>MRLQKDFDRVMGIILMILILAIPSLQICNKSYTEGDPVIINPVPGLPVDFIRGVDASEAPWIIELGGKYYDENGVERDLLDILKENGVNWIRLRVWNDPYDEQGRPYGGGNCDLPRMTDFAAKAKAKGFGVLIDFHYSDWWADPSKQSKPKAWANLSYPELVEAVYNWTYNALKYMAEHNALPDMVQIGNEINNGFLWPDGSAANWTQFVGLLKAAISAVKDVNPNIKIVIHLAGVKADFYINFIDRLINSGVSFDVIAISFYPYWHGTMDDFRNLVRTLVQRYDKKILVAETAYAWTLDDSDGHPNIFGSRDLEVKGGYKASIQGQASFIRDLIAALYEEGKDKALGIFYWGATWIPYPGAGWKTGEGNPWENQALFDFNGRALPSLKVFRLVYEAQPVEIKPLEL[2x]

Endo-β-1,4-galactanases, in particular hydrolyse galactan and arabinogalactan in pectin, a major component of the primary plant cell wall, with important functions in plant defence and application in the food and other industries. Endo-β-1,4-galactanases are glycoside hydrolases (EC 3.2.1.89) that degrade the galactan and arabinogalactan via a double displacement retaining mechanism using two carboxylic acids, one acting as a nucleophile and one functioning as an acid/base. In this article, we thus present the structure and characterization of the hyperthermophilic endo-β-1,4-galactanase catalytic domain from I. aggregans (IaGal). This catalytic domain, obtained from the C-terminal truncation of the full-length gene also encoding an Ig-like and a putative binding domain exhibits a temperature activity optimum of 95 °C making it an asset for future industrial biomass degradation.

As other enzymes in the GH53 family and clan GH-A, the overall structure of IaGal is a (β/α)8 barrel (also known as TIM barrel) which consists of 8 parallel β-sheets (here referred as β1 to β8) and 8 α-helices (here referred as α1 to α8) that alternate along the peptide chain. Loops connecting βn and αn will be referred to the nth β/α-loop. β4 and β7 bear the catalytic acid–base (Glu165) and nucleophile residues (Glu266), respectively. All galactanases structurally characterized to date contain a stabilizing interaction between the 7th and 8th β/α-loop in the (β/α)8 barrel except for BtGal, which has a significantly shorter 7th β/α-loop. The stabilizing interaction has been shown to be a disulphide bridge in all fungal galactanases, and a calcium binding site in BlGal (purple) and now archaeal (green) enzymes. A slight difference is observed in the calcium binding sites between BlGal and IaGal as Glu347 in the archaeal enzyme coordinates both with Oε1 and Oε2, while the corresponding Asp370 in BlGal is angled differently and only coordinates with one oxygen. This results in a coordination number for the calcium ion of 7 in IaGal compared to 6 in BlGal. From the structural point of view, IaGal can be considered an intermediate with respect to substrate binding subsites. The IaGal contains − 1, − 2 and − 3 binding subsites in addition to the + subsites, while the fungal galactanases are devoid of the − 3 subsite and BlGal contains the additional − 4 subsite. Differential scanning calorimetry (DSC) indicated a thermal denaturation midpoint (Tm) of 105 °C for IaGal making it to our knowledge the most thermostable galactanase ever reported. We find that, while salt-bridges and helix stabilization may contribute to IaGal thermostability, H-bonds and compactness do not, and cation–π and π–π interactions are the only features correlating strongly with thermophilicity in GH53 in general.>[2x]MAFELPKLPYAFDALEPHFDKETMEIHHDRHHNTYVTKLNAAVEGTDLESKSIEEIVANLDSVPANIQTAVRNNGGGHLNHSLFWELLSPNSEEKGTVVEKIKEQWGSLEEFKKEFADKAAARFGSGWAWLVVNNGQLEIVTTPNQDNPLTEGKTPILGLDVWEHAYYLKYQNKRPDYIGAFWNVVNWEKVDELYNATK

For example, Staphylococcus aureus has a constitutive Mn-specific superoxide dismutase (herein MnSOD), which is catalytically inactive when loaded with Fe, and a second one (herein camSOD)1 that is stress-induced and cambialistic—that is it can use either Mn or Fe. This cofactor promiscuity enhances the pathogenicity of S. aureus by enabling it to survive the oxidative burst of the innate immune system while experiencing host-imposed Mn starvation. Each monomer presented the characteristic fold conserved amongst Mn/Fe-SODs, with an α-helical N-terminal domain and a C-terminal α/β domain connected by a loop. The active sites were enclosed between the two domains of each monomer, with both domains contributing ligands. As shown in Fig. 3 and as expected, the Mn ions were coordinated in a distorted trigonal bipyramidal geometry by H81, D167, and H171 in the equatorial plane, and H26 and a water molecule in the axial plane.

Preparations of S. aureus MnSOD and camSOD, shown to contain exclusively Mn by ICP-MS, were used in crystallization trials. The crystal structures of Mn(Mn)SOD and Mn(cam)SOD were determined by molecular replacement, using B. subtilis SodA as a search model, at 2.07 Å and 2.30 Å, respectively (data collection and refinement statistics are provided in Table S1, ESI†). Two molecules were found in the asymmetric unit of both protein crystals. The dimers of MnSOD and camSOD were superimposable in the protein backbone with an average root mean square deviation (RMSD) of 0.744 Å by least squares fit. Superposition of equivalent Cα atoms of chain A and chain B of MnSOD and camSOD gave positional RMSDs of 0.232 Å and 0.229 Å, respectively. Most of the differences between the structures were found in the loops connecting helical elements within the N-terminal domains. S. aureus Mn(Mn)SOD and Mn(cam)SOD can be readily distinguished by their 94 GHz field-swept echo EPR spectra. For Mn(Mn)SOD, D = –10.60 and E = 0.63 GHz, similar to E. coli Mn(Mn)SOD; for Mn(cam)SOD, D = –10.66 and E = 0.43 GHz, comparable to the R. capsulatus camSOD; and for Mn(Fe)SOD, D = –10.46 and E = 0.33 GHz, which were the same within errors as those previously obtained from simulations of the Ms = –1/2 ↔ +1/2 transition. In the S. aureus Mn(Mn)SOD, the ring plane of H26 relative to the Mn–Oδ1,Asp167 bond was 180°, while in Mn(cam)SOD it was 167°. The 94 GHz ELDOR-NMR and ENDOR of Mn(Mn)SOD and Mn(cam)SOD are remarkably similar, indicating a high-degree of structural homology even at the level of the positions of the protons in proximity to the metal ion, in particular those of the water ligand.>GPGSMGRVQDKVVLVTGGARGQGRSHAVKLAEEGADIILFDICHDIETNEYPLATSRDLEEAGLEVEKTGRKAYTAEVDVRDRAAVSRELANAVAEFGKLDVVVANAGICPLGAHLPVQAFADAFDVDFVGVINTVHAALPYLTSGASIITTGSVAGLIAAAQPPGAGGPQGPGGAGYSYAKQLVDSYTLQLAAQLAPQSIRANVIHPTNVNTDMLNSAPMYRQFRPDLEAPSRADALLAFPAMQAMPTPYVEASDISNAVCFLASDESRYVTGLQFKVDAGAMLKF[6x]

Here we present a series of TIGR03971 SDR crystal structures from several mycobacterial species which contain an insertion in the primary sequence at the NAD cofactor binding site. These crystal structures demonstrate that the inserted protein residues almost completely cover the NAD cofactor, only leaving part of the nicotinamide ring exposed to solvent. NMR experiments did not show exchange of the NAD cofactor, whereas binding was demonstrated for a number of small molecules which could be potential substrates, products, inhibitors, or artificial redox partners. Experimental results are consistent with the notion that the SDR family enzymes linked by comparative genomics studies to mycofactocin do indeed keep their NAD tightly bound beneath a protein structure that may interact with a specialized adaptor machinery for redox exchange.

With the exception of the M. thermoresistibile target which did not contain NAD, all other mycobacterial SDR target crystal structures contained NAD, which appears to have co-purified with the protein after expression in E. coli. For each of these crystal structures, the adenosine mononucleotide portion of the cofactor binding site is enveloped by the inserted residues and only a portion of the nicotinamide ring appears open to solvent (see representative examples in Fig. 2A and B). In addition to the insertion loop which covers the adenosine portion of the cofactor, a second loop which typically contains two α-helices covers much of nicotinamide mononucleotide portion of the cofactor. In contrast, this loop is ordered in each of the mycobacterial SDR crystal structures presented here. The combination of the insertion loop which covers the adenosine portion of the cofactor and the ordering of the second loop which covers the nicotinamide mononucleotide portion of the cofactor results in a significant decrease in the solvent accessible surface area of the cofactor in the mycobacterial SDRs, relative to other NAD- and NADP-dependent dehydrogenases. Only a small portion of the nicotinamide ring appears available to solvent in each of these cases, indicating that the NAD cofactor is tightly bound and potentially non-exchangeable. The structures presented here have a cofactor solvent accessible surface area of approximately 18 Å2, whereas other NAD- or NADP-bound dehydrogenases have a cofactor solvent accessible surface area of 82–89 Å2. Given the encapsulation of the NAD cofactor by the two loops in mycobacterial SDRs, a large conformational change would be required to release the NADH cofactor after a redox reaction had occurred. To test whether or not the bound NAD was exchangeable, we performed a number of line broadening and STD-NMR ligand-observe studies, and did not observe exchange of NAD/NADH during the timescale of the NMR experiments.>[2x]GSHMTAYTAERQPERDITPVNDETMQE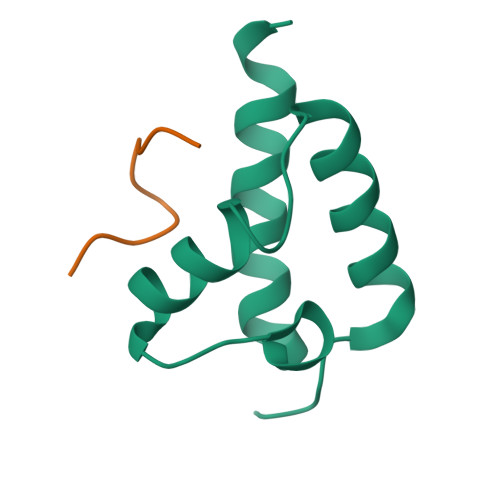INTLLIALDKTWDDDLLPLCSQIFRRDIRASSELTQAEAVKALGFLKQKAAEQKVAA;>WMDFDDDIPF[2x]>MGHHHHHHMDKKPLNTLISATGLWMSRTGTIHKIKHHEVSRSKIYIEMACGDHLVVNNSRSSRTARALRHHKYRKTCKRCRVSD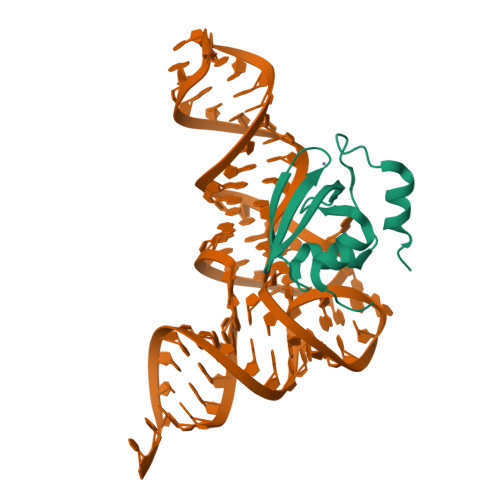EDLNKFLTKANEDQTSVKVKVVSAP[2x]> VVNGIPTRTNIGWMVSLRYRNKHICGGSLIKESWVLTARQCFPSRDLKDYEAWLGIHDVHGRGDEKCKQVLNVSQLVYGPEGSDLVLMKLARPAVLDDFVSTIDLPNYGSTIPEKTSCSVYGWGYTGLINYDGLLRVAHLYIMGNEKCSQHHRGKVTLNESEICAGAEKIGSGPCEGDYGGPLVCEQHKMRM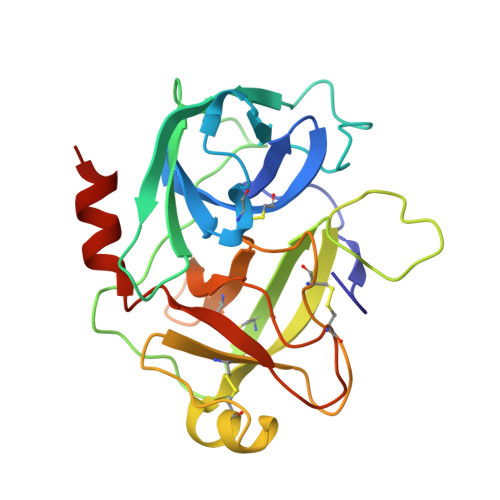VLGVIVPGRGCAIPNRPGIFVRVAYYAKWIHKIILTYKVPQS>MNLKPQTLMVAIQCVAARTRELDAQLQNDDPQNAAELEQLLVGYDLAADDLKNAYEQALGQYSGLP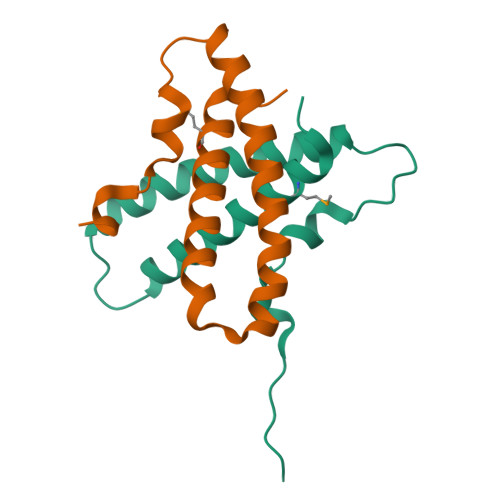PYDRLIEEPASLEHHHHHH[2x]> GHMMSQSNRELVVDFLSYKLSQKGYSWSQFSDVEENRTEAPEGTESEAVKQALREAGDEFELRYRRAFSDLTSQLHITPGTAYQS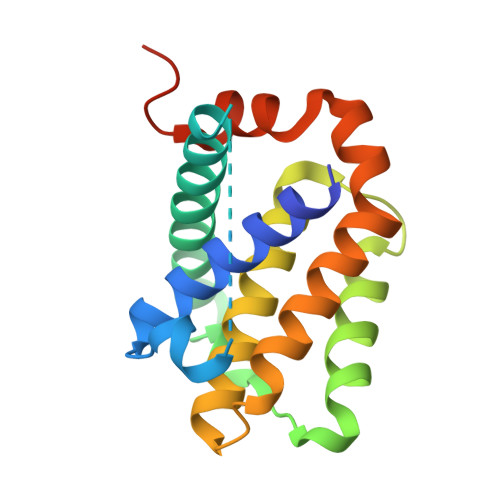FEQVVNELFRDGVNWGRIVAFFSFGGALCVESVDKEMQVLVSRIAAWMATYLNDHLEPWIQENGGWDTFVELYGNNAAAESRKGQER> GAMDKRTQPTTGTSGGYYFSFWTDTPNSVTYTNGNGGQFSMQWSGNGNHVGGKGWMPGTSRTIKYSGSYNPNGNSYLAVYGWTRNPLIEYYIVENFGTYNPSSGGQKKGEVNVDGSVYDIYVSTRVNAPSIDGNKTFQQYWSVRRNKRSSGSVNTGAHFQAWKNVGLNLGTHDYQILAVEGYYSSGSASMTVSQ

Here, we describe the crystal structure and enzymatic properties of Xyl2, a novel GH11 endo-β-1,4-xylanase from the pathogenic fungus F. oxysporum that also exhibits a synergic β-d-xylosidase activity. Overall, Xyl2 folds into the characteristic GH11 xylanase fold consisting of a highly twisted β-sandwich core that comprises 14 β-strands and is further stabilized by a single α-helix in the opposite side of the active site. The groove delimited by the long β-hairpin, commonly denominated the “thumb” region, and the curved side of the β-sandwich or “fingers” region defines a long, wide valley into which the xylan substrate molecule binds, or “palm” region. The general mechanism of glycoside hydrolases (GH) starts with the nucleophilic attack by a carboxylate nucleophile (Glu176 side chain) on the anomeric carbon of the scissile glycosidic bond, resulting in the release of the linked sugar residue and the formation of a covalent enzyme–sugar intermediate.

The crystal structure of Xyl2 at 1.56 Å has revealed an atomic-level view of the active-site groove from which the catalytic mechanism can be inferred. The final model contains the complete amino acid sequence except for the first and last amino acids (residues 2-190). The N-terminus of Xyl2, however, adopts a particular conformation and, instead of running away from the active site, it folds into an elongated motif that forms one side of the active-site groove. Since the position and orientation of this unique feature appear to complete the fingers in Xyl2, we propose to call this unique feature the “pinky” motif. Besides Tyr76, the residues in the active site from the palm region (Tyr179, Gln136, Arg121 and Asn70) are fully conserved across GH11 xylanases and entirely defined in the electron density map at 1.56 Å contoured at 1σ level. Comparison of the Xyl2/MBX and the unliganded Xyl2 active-site structures revealed that, in the unliganded Xyl2, a glycerol molecule from the cryoprotectant solution was found in the active site near to the position occupied by MBX ligand. The glycerol molecule is stabilized by interactions with the side chains of the catalytic residues Tyr87, Arg121 and Gln135, and is well defined in the electron density map, which reinforces the view that Xyl2 active site is particularly capable of binding xylose and chemically related molecules situated at position-2, the position of the xylene subunit immediately adjacent to the β-(1,4) glycosidic bond to be hydrolyzed. In the observed conformations, Glu176 side chain points to the bulk solvent, which causes the side chain of Tyr72 to concertedly flip over to a less hindered conformation. The present structure confirms the poor activity for Xyl2 at this pH since it presents a concerted change in the Glu176 and Tyr72 rotamers, with the nucleophilic Glu176 side chain being kept away from the substrate.>MSKEVSEEAQAHQHGKDYVDPPPAPFFDLGELKLWSFWRAAIAEFIATLLFLYITVATVIGHSKETVVCGSVGLLGIAWAFGGMIFVLVYCTAGISGGHINPAVTFGLFLARKVSLLRALVYMIAQCLGAICG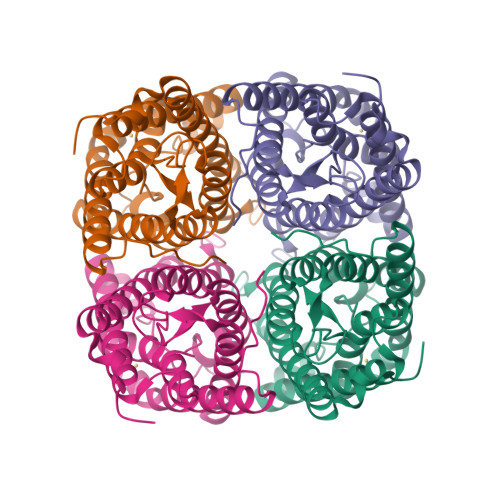VGLVKAFMKGPYNQFGGGANSVALGYNKGTALGAEIIGTFVLVYTVFSATDPKRSARDSHVPILAPLPIGFAVFMVHLATIPITGTGINPARSFGAAVIFNSNKVWDDQWIFWVGPFIGAAVAAAYHQYVLRAAAIKALGSFRSNPTN[2x]>LSTSLSALPAAARDFVEEAVRLCR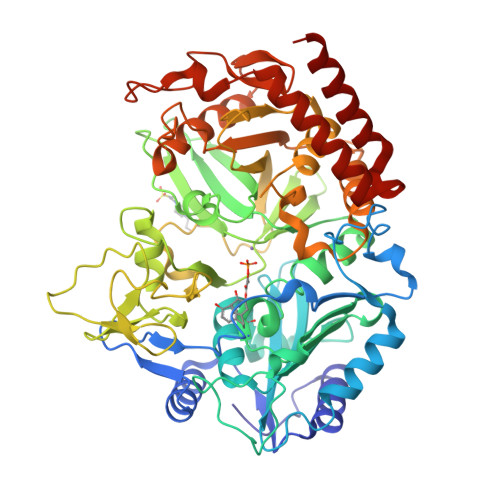PREVLLCDGSEEEGKELLRGLQDDGVLHPLPKYDNCWLARTDPRDVARVESKTVLVTPEQSDAVPPPPPSGGPPQLGNWMSPNAFQAAVQERFPGCMAGRPLYVIPFSMGPPTSPLAKLGVQVTDSPYVVLSMRIMTRVGPAVLQRLDDDFVRCLHSVGRPLPLTEPLVSSWPCDPSRVLVAHIPSERRIVSFGSGYGGNSLLGKKCFALRIASRMAQQQGWLAEHMLILGVTSPSGEKRYMAAAFPSACGKTNLAMMTPSLPGWRIHCVGDDIAWMKFDDEGRLRAINPERGFFGVAPGTSSRTNPNAMATIARNTIFTNVGLRSDGGVYWDGLDEPTEPGVTYTSWLGKPWKHGDPEPCAHPNSRFCAPADQCPIMDPRWDDPEGVPIDAIIFGGRRPRGVPLVVEAFGWRHGVFMGSAMRSEATAAAEHKGGRLMHDPFAMRPFFGYNAGRYLEHWLSTGLRSNARLPRLFHVNWFLRDNEGRFVWPGFGHNARVLAWIFGRIQGRDTARPTPIGWVPKEGDLDLGGLPGVDYSQLFPMEKGFWEEECRQLREYYGENFGADLPRDVMAELEGLEERVRKM[2x]> MHHHHHHMKDFIKEFLNERPEVV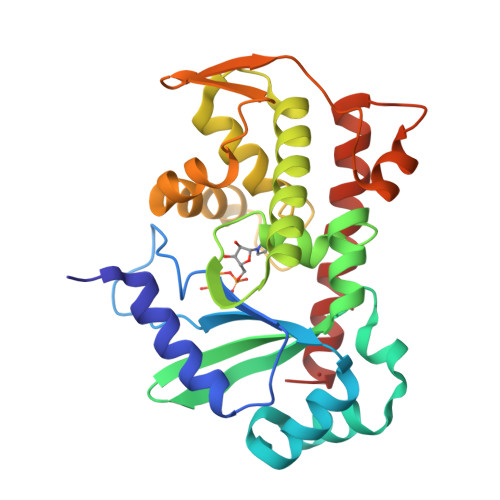AAFGYGSGVFKQLGYDSKEKPQIDLILIVNDMKLWHKENIKKNPKDYSFIGRNFFLNSSIDEIKGITGITYQSNIEYKGHLFKYGIIEYGDFVRHMQTWDSFYVPGRFQKPILTIKSNNFIDELILQNRRNACKVGLLCLNNKDLKDLYLTICNLSYSGDTRMKVAENPKKVENIVGASYDKFNEMYNFNDLYQKNGERIEYEIDIDELPSSLEKYIKDDKTKEKVMEYLSDLNRKESSLQTMKGIKTN(3E)-4-{3-HYDROXY-2-METHYL-5-[(PHOSPHONOOXY)METHYL]PYRIDIN-4-YL}-2-IMINOBUT-3-ENOIC 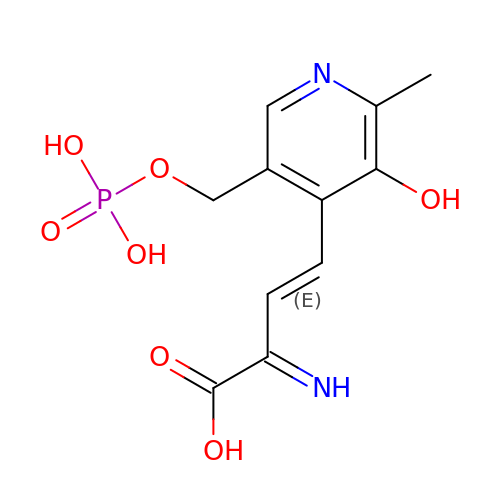ACID | C11 H13 N2 O7 P | RFCLOBQLGFQJHL-LDEIZCIFSA-N>[6x]MDSFSANQEIRYSEVTPYHVTSVWTKGVTPPANFTQGEDVFHAPYVANQGWYDITKTFNGKDDLLA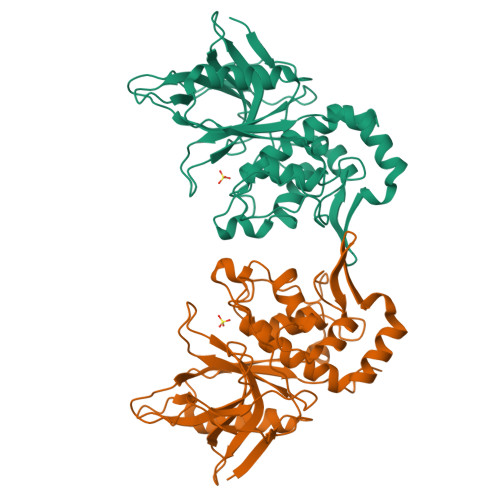GAATAGNMLHWWFDQNKDQIKRYLEEHPEKQKINFNGEQMFDVKEAIDTKNHQLDSKLFEYFKEKAFPYLSTKHLGVFPDHVIDMFINGYRLSLTNHGPTPVKEGSKDPRGGIFDAVFTRGDQSKLLTSRHDFKEKNLKEISDLIKKELTEGKALGLSHTYANVRINHVINLWGADFDSNGNLKAIYVTDSDSNASIGMKKYFVGVNSAGKVAISAKEIKEDNIGAQVLGLFTLSTGQDSWNQTN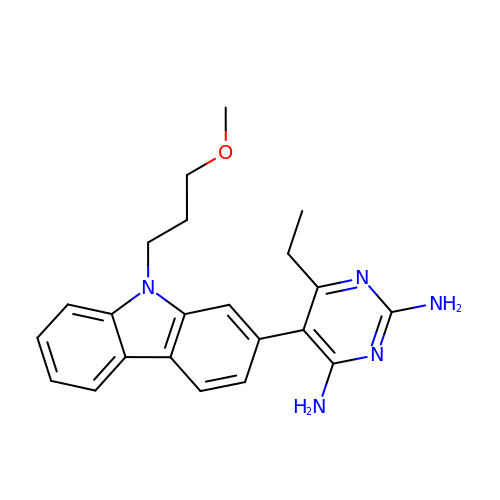6-ETHYL-5-[9-(3-METHOXYPROPYL)-9H-CARBAZOL-2-YL]PYRIMIDINE-2,4-DIAMINE | C22 H25 N5 O | MLSVRCGEBXIIQO-UHFFFAOYSA-N> MPGAISQLVSYGAQDVYLTGNPQITFFKAVYRRYTNFAMESIQQTFDGTTDFGKFPTVTISRNGDLAGPIWIEVNLPSLLGYNITPTPAEGNTSNIAAISTVFKDDYNNYWWTYNPGTTPQYSNLIAAFSNVDYKYYANAVTSTYPPTALSNVVYSWPYMITGNTGTRSTVAIPTANLRYVNGIGLALFNSIELELGGQRIDKHYSEWWDIWTELTETAEKIQGYNTMVGRYDPAVYNAGWNISQA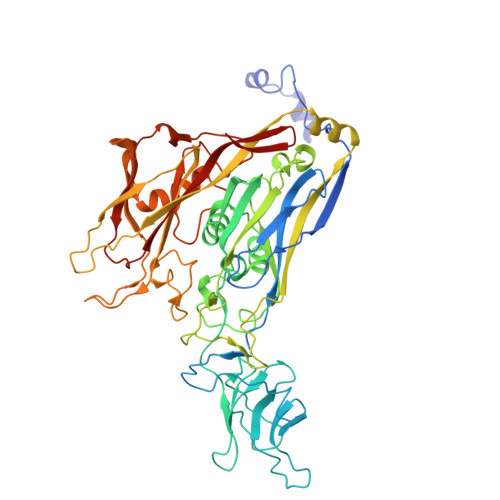QGGTYYVPLKFCYNRNPGLYMPLVALSYHQMKLNFNINNYLNCVKCNYPVTALTSKNGANPLSITNMKLYTDFVFLDAPERIRMSEIQHEYLVTQLQWQGSEPVTAPGDPNGSTNRKITLNFNHPVRELVFVYQAASNYDVDAVTGNNIFDYEIPANPTATPPYAGGGEVFTEVKLIINGSDRFSGRPGAYFRLVQPYEHHVRVPSKSVYVYSFALEDADSRQPNGSANFTRYDSVQLQLTLNENLASGRVQIYAPNFNILRIAAGMGGLAFAN> EEMKKGHLERECMEETCSYEEAREVFEDSDKTNEFWNKYKDGDQCETSPCQNQGKCKDGLGEYTCTCLEGFEGKNCELFTRKLCSLDNGDCDQFCHEEQNSVVC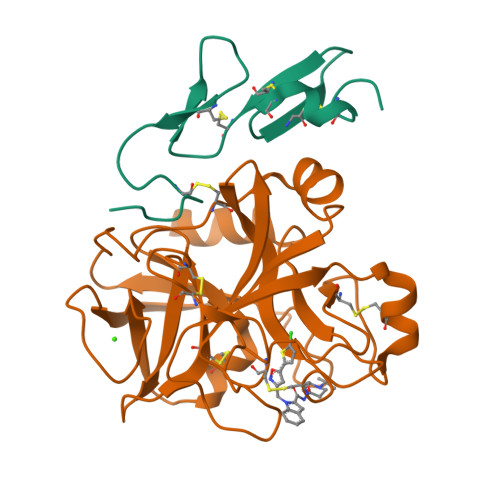SCARGYTLADNGKACIPTGPYPCGKQTLER;> IVGGQECKDGECPWQALLINEENEGFCGGTILSEFYILTAAHCLYQAKRFKVRVGDRNTEQEEGGEAVHEVEVVIKHNRFTKETYDFDIAVLRLKTPITFRMNVAPACLPERDWAESTLMTQKTGIVSGFGRTHEKGRQSTRLKMLEVPYVDRNSCKLSSSFIITQNMFCAGYDTKQEDACQGDSGGPHVTRFKDTYFVTGIVSWGEGCARKGKYGIYTKVTAFLKWIDRSMKTRGLPKAKSHAPEVITSSPLK1-chloranyl-3-methylsulfinyl-6,7-dihydro-5H-2-benzothiophen-4-one | C9 H9 Cl O2 S2 | 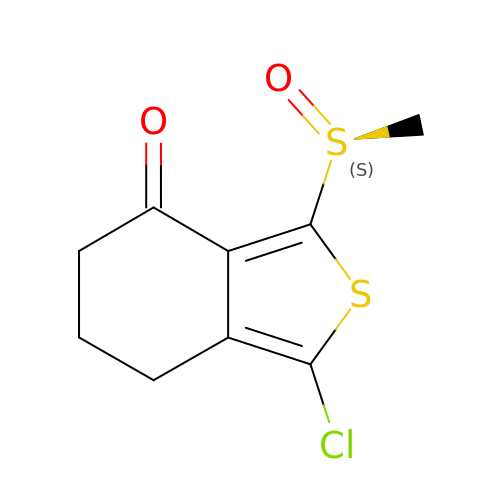PGSSJIDFZJTWLZ-AWEZNQCLSA-N Lipin/Pah phosphatidic acid phosphatases (PAPs) are Mg2+-dependent enzymes that catalyze the dephosphorylation of phosphatidic acid (PA) to produce diacylglycerol. pmcLipin/Pah phosphatidic acid phosphatases (PAPs) are magnesium-dependent enzymes that are evolutionarily conserved from yeast to humans. They catalyze the penultimate step of triacylglycerol synthesis, through the conversion of phosphatidic acid (PA) to diacylglycerol (DAG). Structurally, all lipin/Pah PAPs contain highly conserved N-Lip and C-Lip regions that combine to form two domains: an immunoglobulin-like (Ig-like) domain and a HAD-like catalytic domain. The remainder of the C-Lip adopts a Rossmann-fold, forming the haloacid dehalogenase-like (HAD-like) domain and harbors a conserved catalytic motif DxDxT, where the first Asp coordinates a Mg2+ ion that increases its nucleophilicity, and the second Asp participates in acid/base catalysis.

Structures 2, 3, and 4 were determined using a Δhelix construct with a D148N point mutant that modified the DxDxT motif to be DxNxT. Mutating polar residues in the active site to nonpolar equivalent residues has been demonstrated to stabilize HAD phosphatases, enhancing structure resolution. The Δhelix D148N point mutant was crystallized in an apo state, Mg2+-bound, and Mg2+ tungstate-bound states by crystal soaking. The Δhelix D148N structures were crystallized without any cofactors and then soaked with either magnesium, or magnesium and tungstate to generate three structures with active sites in distinct states. Comparison of the apo and magnesium bound structure saw replacement of a water molecule with a hexa-coordinated magnesium ion in the active site, characteristic of a HAD phosphatase. The sixth and final magnesium coordination site was occupied by the carboxylic acid group from the sidechain of Asp155 and was located distal to the catalytic Asp146 on the opposite side of the magnesium ion. In the apo structure, Asp155 was observed in a similar conformation but coordinated the water molecule in place of the magnesium. To determine structures of additional catalytic states, we soaked Δhelix D148N apo crystals with magnesium and a variety of substrates and transition state analogs.

> SFSGVVDIIVVRQPDDSLKSMPFHIRFGTLKVLDNQNINIQITVNDKKIEDVFMLMLPEGACYFPELNAKNEIQKKLRPSSAILKKFNLKNGYNKIQFIAESDLQGKQLIEGKIYLYNYDTKLVISDVNGTVTKSDVKGHISTIIGKEWTHDDIAELYTNIQKNGYKMVYLSSRPLYFYNYTQGYLKGIIQNGFTMPDGPILLSPDQIISSLNREVVYKKADEFKGALLKDLRRVFPEEVNPIFAGFGNRDTDATACLYAGVIIDNIFIINEQSQVEILGKQEKSSYKKINEKIQELFPRLP> MPTPSHLKNPLCFDFRAARRVPETHAWPGLDDHPVVDGGGG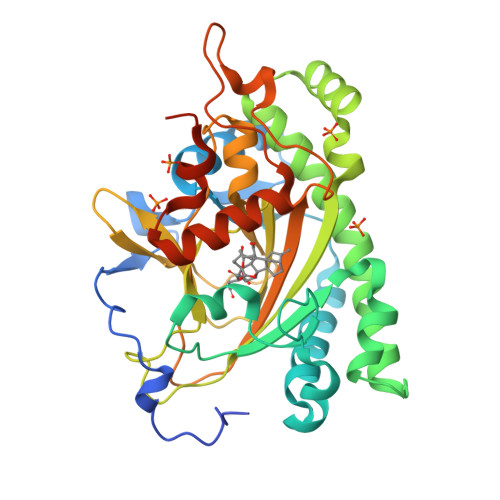GGEDAVPVVDVGAGDAAARVARAAEQWGAFLLVGHGVPAALLSRVEERVARVFSLPASEKMRAVRGPGEPCGYGSPPISSFFSKLMWSEGYTFSPSSLRSELRRLWPKSGDDYLLFCDVMEEFHKEMRRLADELLRLFLRALGLTGEEVAGVEAERRIGERMTATVHLNWYPRCPEPRRALGLIAHTDSGFFTFVLQSLVPGLQLFRRGPDRWVAVPAVAGAFVVNVGDLFHILTNGRFHSVYHRAVVNRDRDRVSLGYFLGPPPDAEVAPLPEAVPAGRSPAYRAVTWPEYMAVRKKAFATGGSALKMVSTDAAAAADEHDDVAAAADVHA>[4x]TIIINVRERIEEWKIRIAA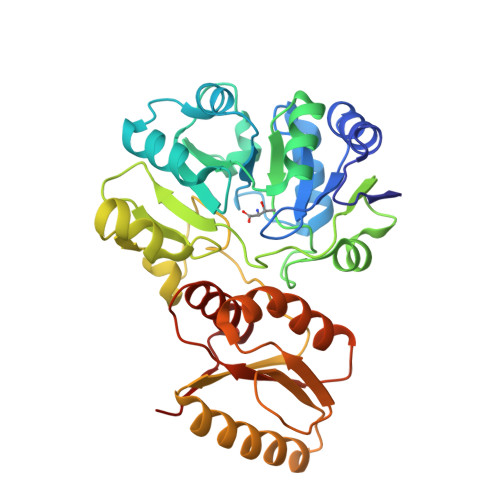GFIREGKLVAFPTETVYGLGANALDENAVKRIFEAKGRPADNPLIIHIASFEQLEVLAKEIPEEAEMLAKRFWPGPLTLVLPKSEVVPRVITGGLDTVAVRMPAHEIALKLIELSERPIAAPSANISGKPSPTSAHHVAEDFYGKIECIIDGGETRIGVESTVIDLTEWPPVLLRPGGLPLEEIEKVIGEIRIHPAVYGKSVDTAKAPGMKYRHYAPSAEVIVVEGPRDKVRRKIEELIAKFKEEGKKVGVIGSGSYDADEVFYLGDTVEEIARNLFKALRHMDRTGVDVILAEGVEEKGLGLAVMNRLRKASGYRIIKVHHHHHH>[2x]MSSVLVLGRISDDPASHYEQLKPLLDYVVPRMREVGIRRGEILMAPDARQMSSY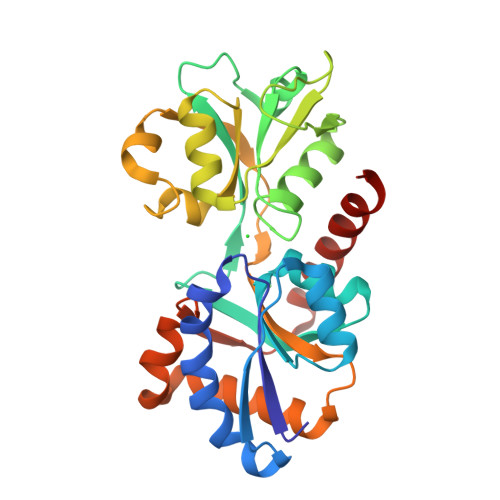LRRGRVDWVSETTGAAMLLEQRGSAHPLLMTERGGLRDFHTLFFVRRDSPIHSLSQLRGHTLALQNASSTSGYLLPMLELLRNGIACDVLLSADDTPARGSAGYLMVGSKLNVAAFVHKHLIDVGALSNVDWDDERHMPPVFKRDFRIVHRTAPVPRAVEMVRTGMDPAVEQRLRVVLLQAASDPKAGPALKRFFDTTGFRPLDPTSRRRLQELSAGVQRVRDHVE>MPITLYSVSDGPPSLAVRQALEYLGLEHKLVNVDFGIGEHMTEEFAQKNPQKEIPVLDDNGFLLGESNAILQYLAERYGKDDTIYPKDPMARAVVNHRLCFNLSTYYRYISEYTLAPMFFDYQRTPLGLKKTHIALDNFNTYLKLLGKKYAAGET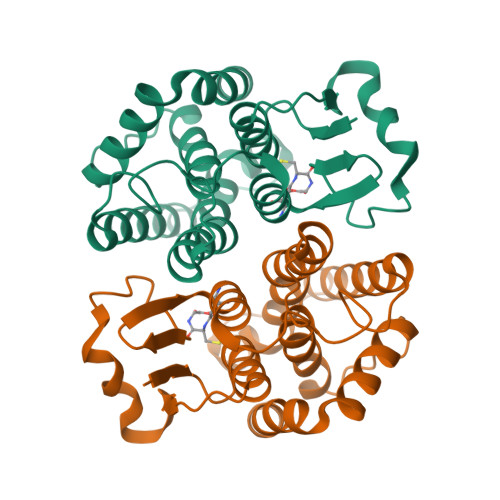VTIADFQLVTATMCLEAINFDISPWPLVENWYDTYKLEHPTLWKIVEGGMKELEAFEKNPPDLSHMDHPIHPVRK[2x]> MILDTDYITEDGKPVIRIFKKENGEFKIDYDRNFEPYIYALLKDDSAIEDVKKITAERHGTTVRVVRAEKVKKKFLGRPIEVWKLYFTHPQDVPAIRDKIKEHPAVVDIYEYDIPFAKRYLIDKGLIPMEGDEELKMLAFDIETLYHEGEKFAEGPILMISYADEEGARVITWRNIDLPYVDVVSTEKEMIKRFLKVVKEKDPDVLITYNGDNFAFAYLKKRSEKLGVKFILGREGSEPKIQRMGDRFAVEVKGRIHFDLYPVIRRTINLPTYTLEAV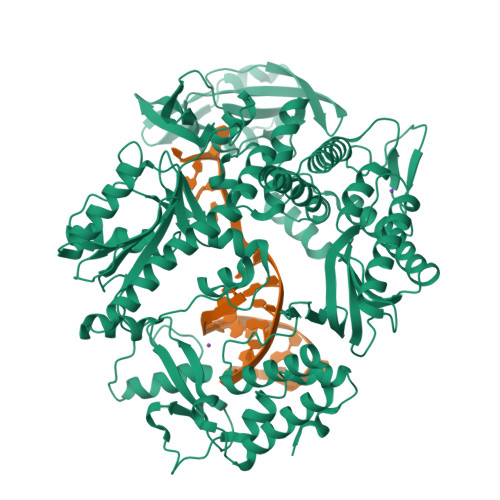YEAIFGQPKEKVYAEEIAQAWETGEGLERVARYSMEDAKVTYELGKEFFPMEAQLSRLVGQSLWDVSRSSTGNLVEWFLLRKAYERNELAPNKPDERELARRRESYAGGYVKEPERGLWENIVYLDFRSLYPSIIITHNVSPDTLNREGCEEYDVAPQVGHKFCKDFPGFIPSLLGDLLEERQKVKKKMKATIDPIEKKLLDYRQRAIKILANSFYGYYGYAKARWYCKECAESVTAWGRQYIETTIREIEEKFGFKVLYADTDGFFATIPGADAETVKKKAKEFLDYINAKLPGLLELEYEGFYKRGFFVTKKKYAVIDEEDKITTRGLEIVRRDWSEIAKETQARVLEAILKHGDVEEAVRIVKEVTEKLSKYEVPPEKLVIYEQITRDLKDYKATGPHVAVAKRLAARGIKIRPGTVISYIVLKGSGRIGDRAIPFDEFDPAKHKYDAEYYIENQVLPAVERILRAFGYRKEDLRYQKTRQVGLGAWLKPKT7-methoxy-~{N}-[(3~{S})-1-(4-methylphenyl)pyrrolidin-3-yl]-1~{H}-indole-3-carboxamide | C21 H23 N3 O2 | 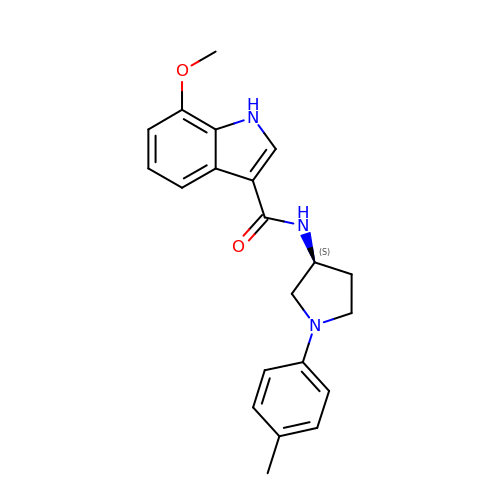GMGMKERXGPBQDO-HNNXBMFYSA-N>MLSYRHSFHAGNHADVLKHTVQSLIIESLKEKDKPFLYLDTHAGAGRYQLGSEHAERTGEYLEGIARIWQQDDLPAELEAYINVVKHFNRSGQLRYYPGSPLIARLLLREQDSLQLTELHPSDYPLLRSEFQKDSRARVEKADGFQQLKAKLPPVSRRGLILIDPPYEMKTDYQAVVSGIAEGYKRFATGIYALWYPVVLRQQIKRMIHDLEATGIRKILQIELAVLPDSDRRGMTASGMIVINPPWKLEQQMNNVLPWLHSKLVPAGTGHATVSWIVPESKGHHHHHH[2x]

Nucleotide A2030, the modification site of RlmJ, is located in the hairpin loop of helix 72 (H72) at the 5′ boundary of domain V in 23S rRNA. The RlmJ structure consists of a discontinuous MTase domain (residues 1–46 and 99–280), interrupted by a helical subdomain (HS, residues 47–98). The structure of RlmJ is the first one of an enzyme with demonstrated monomethylating m6A RNA MTase activity. There was no detectable MTase activity on any of the mutant RNAs or the single-stranded DNA. These data show RlmJ is highly specific to adenosine at position 2030, requiring only a small hairpin for activity.

The RlmJ structure was solved in space group P21 with two monomers in the asymmetric unit related by a 2-fold non-crystallographic symmetry. The structure suggests that RlmJ functions as a monomer, consistent with its behavior in size exclusion chromatography. The final models consist of residues 2–280, but with residues 53–55 missing in the second molecule. An extra helix α9 and strand β10 at the C-terminal end of RlmJ distinguishes it from the canonical class I Rossmann-like MTase fold. The location of the inserted subdomain is novel among AdoMet-dependent MTases. Comparison of the structures shows that one molecule in the RlmJSAM structure has the same conformation as the RlmJAPO structure, whereas the other molecule takes the conformation of the RlmJSAH-AMP structure [root mean square deviation (RMSD) of 0.2 Å over 280 Cα atoms for the respective comparison]. In the open form, motif X does not approach the active site, and instead is stabilized by interactions with strand β2 (R47 and Q49) and helix α5 (residues D123–E130).3-(P-TOLYL)PROPIONIC 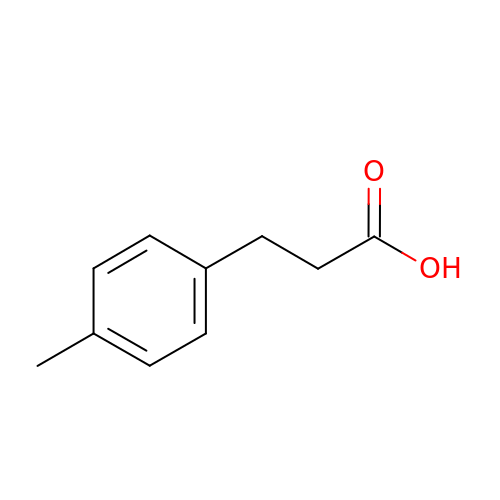ACID | C10 H12 O2 | LDYGRLNSOKABMM-UHFFFAOYSA-N> PYAGSTDE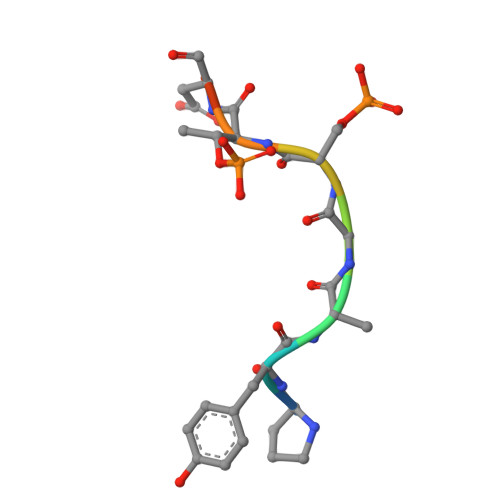N> VVRVADTMPSGPSNSESIPALTAAETGHTSQVVPSDTIQTRHVRNFHVRSESSVENFLSRSACVYIVEYKTRDDTPDKMYDSWVINTRQVAQLRRKLEFFTYVRFDVEVTFVITSVQDDSTRQNTDTPALTHQIMYVPPGGPIPQAVDDYNWQTSTNPSVFWTEGNAPPRMSIPFMSVGNAYSNFYDGWSHFSQTGVYGFNTLNNMGKLYFRHVNDKTISPITSKVRIYFKPKHVKAWVPRPPRLCEYTHKDNVDFEPKGVTTSRTQLTISNSTHVEN;> SDRVRSITLGNSTITTQESANVVVGYGVWPDYLSDEEATAEDQPTQPDVATCRFYTLDSVSWMKESQGWWWKFPDALRDMGLFGQNMQYHYLGRSGYTIHVQCNASKFHQGCLLVVCVPEAEMGAANINEKINREHLSNGEVANTFSGTKSSNTNDVQQAVFNAGMGVAVGNLTIFPHQWINLRTNNCATIVMPYIN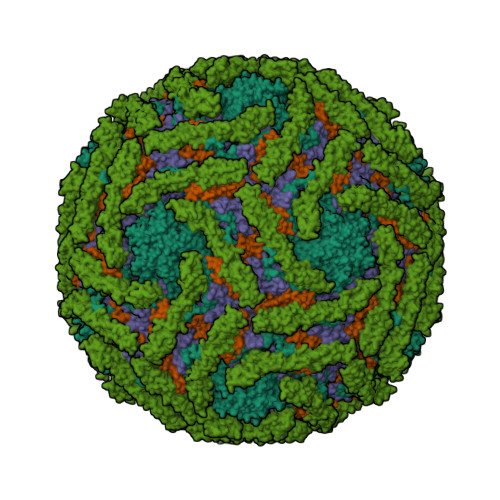SVPMDNMFRHYNFTLMIIPFAKLDYAAGSSTYIPITVTVAPMCAEYNGLRLAGHQ;> GLPVMNTPGSNQFLTSDDYQSPTAMPQFDVTPEMNIPGEVKNLMEIAEVDSVVPVNNVNENVNSLEAYRIPVHSVTETGAQVFGFTLQPGADTVMERTLLGEILNYYANWSGSIKLTFMYCGSAMATGKFLLAYSPPGAGVPKNRREAMLGTHIIWDIGLQSSCVLCVPWISQTHYRFVSKDIYTDAGFITCWYQTSIVVPAEVQNQSVILCFVSACNDFSVRLLRDSPFVRQTAFYQ;> GAQVSTQKTGAHETSLSASGNSIIHYTNINYYKDAASNSANRQDFTQDPGKFTEPVKDIMVKSLPALN;> CNRSCEVPTRLNSASLKQPYITQNYFPVGTVVEYECRPGYRREPSLSPKLTCLQNLKWSTAVEFCKKKSCPNPGEIRNGQIDVPGGILFGATISFSCNTGYKLFGSTSSFCLISGSSVQWSDPLPECREIYCPAPPQIDNGIIQGERDHYGYRQSVTYACNKGFTMIGEHSIYCTVNNDEGEWSGPPPECRG> GEEIKETFEVDDLDEALRLSAEKIIEEMKKWGVTEFD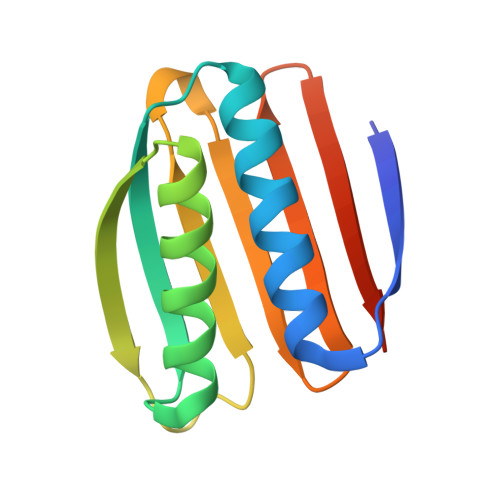LKFYGKDDELAKKAKEVIEEAAKKAGVKVKSEFLYDENKDKITLELTGPNGVKVTSEISKDGIKSTVERPDRKVTLTFKLEHHHHHH>ARQERAAQTRRTIVAAAAAVFDELGYEATTIAEILKRSGVTKGALYFHFTSKEQLAQEVLTSQLRAVPPVEEQRLVLQQIIDETLLLAQLLSKGDPLVRGSVRLTVEPGAPADGLDRRAPMQEWIGHGRDLLRRAEAGGELLPRLDVDAVARMLVGGFTGAQILSNILTGHADLLERVTDMHRHLMTSVAVPAVLVRLDFSAERSITVYDEAMRRREAPLPAAGDLEH[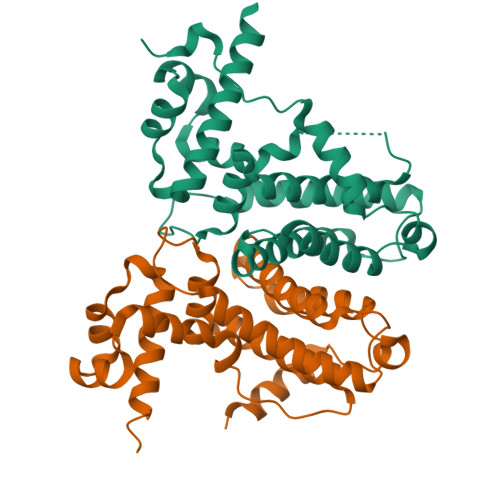8x]>[4x]DRHHHHHHKLIGEGASRDDDLLVPYPRARLRPVRDCTPVHTGSLKHENWPPPPAAPGAGPPAVRTFVSHFGGRAVSGHLTRAAAPLRTFSV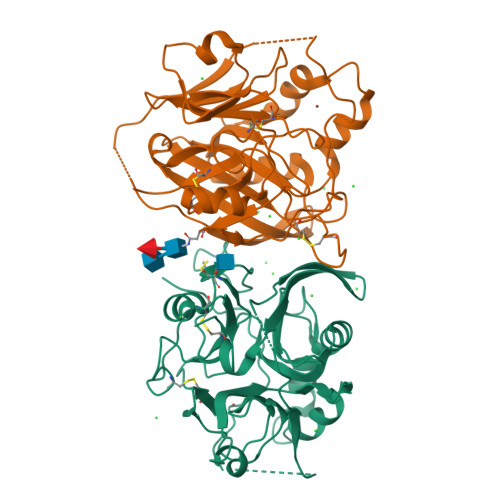LEPGGPGGCSQKRRATVEETAQAAACRIAQNGGFFRMNTGECLGNVVSDGRRVSSSGGLQNAQFGIRRDGTLVTGYLSEEEVLDTENPFVQLLSGVVWLIRNGSIYINESQATECDETQETGSFSKFVNVMSARTAIGHDRDGQLVLFHADGQTEQRGINLWEMAEFLLRQGVVNAINLDGGGSATFVLNGTLASYPSDHCQDNMWRCPRRVSTVVCVHEP> MPSRVPKSIFYNQVGYLISGDKRFWIQAHEPQPFALRTPEGQAVFAGMTKPVGGNWYVGDFTALRVPGTYTLTVGTLEARVVIHRRAYRDVLEAMLRFFDYQLCGVVLPEDEAGPWAHGACHTSDAKVFGTERALACPGGWHDAGDYGKYTVPAAKAVADLLLAHEYFPAALAHVRPMRSVHRAPHLPPAL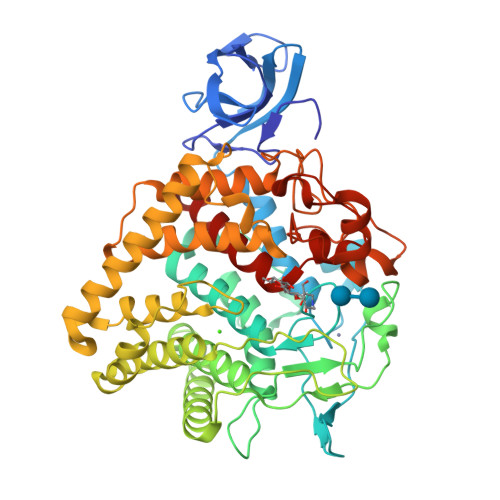EVAREEIAWLLTMQDPATGGVYHKVTTPSFPPLDTRPEDDDAPLVLSPISYAATATFCAAMAHAALVYRPFDPALSSCCADAARRAYAWLGAHEMQPFHNPDGILTGEYGDAELRDELLWASCALLRMTGDSAWARVCEPLLDLDLPWELGWADVALYGVMDYLRTPRAAVSDDVRNKVKSRLLRELDALAAMAESHPFGIPMRDDDFIWGSNMVLLNRAMAFLLAEGVGVLHPAAHTVAQRAADYLFGANPLGQCYVTGFGQRPVRHPHHRPSVADDVDHPVPGMVVGGPNRHLQDEIARAQLAGRPAMEAYIDHQDSYSTNEVAVYWNSPAVFVIAALLEARGR>[7x]GSVIDVSSQRVNVQRPLDALGNSLNSPVIIKLKGDREFRGVLKSFDLHM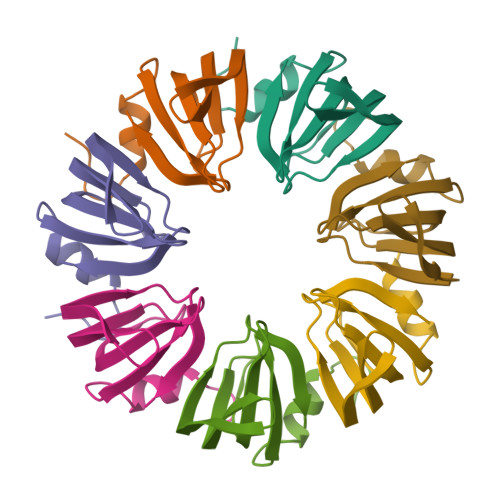NLVLNDAEELEDGEVTRRLGTVLIRGDNIVYISP> QSSVTLFGIVDTNVAYVNKDAAGDSRYGLGTSGASTSRLGLRGTEDLGGGLKAGFWLEGEIFGDDGNASGFNFKRRSTVSLSGNFGEVRLGRDLVPTSQKLTSYDLFSATGIGPFMGFRNWAAGQGADDNGIRANNLISYYTPNFGGFNAGFGYAFDEKQTIGTADSVGRYIGGYVAYDNGPLSASLGLAQQKTAVGGLATDRDEITLGASYN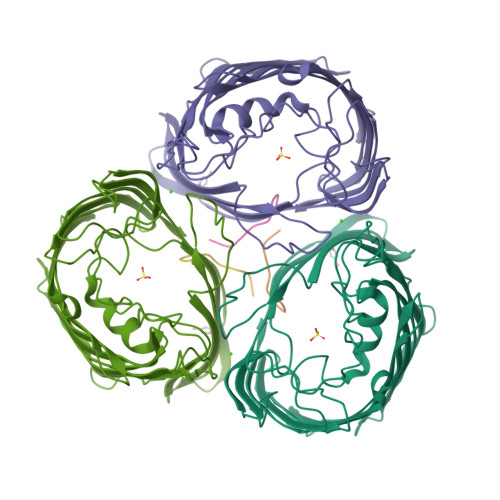FGVAKLSGLLQQTKFKRDIGGDIKTNSYMLGASAPVGGVGEVKLQYALYDQKAIDSKAHQITLGYVHNLSKRTALYGNLAFLKNKDASTLGLQAKGVYAGGVQAGESQTGVQVGIRHAF;> DNWQNGTS>[30x]MSMYTTAQLLAANEQKFKFDPLFLRLFFRESYPFTTEKVYLSQIPGLVNMALY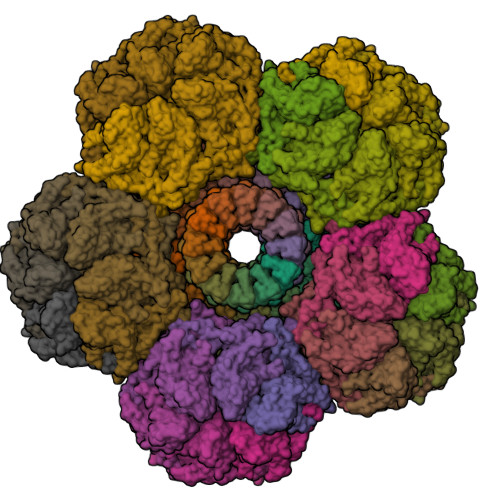VSPIVSGEVIRSRGGSTSEFTPGYVKPKHEVNPQMTLRRLPDEDPQNLADPAYRRRRIIMQNMRDEELAIAQVEEMQAVSAVLKGKYTMTGEAFDPVEVDMGRSEENNITQSGGTEWSKRDKSTYDPTDDIEAYALNASGVVNIIVFDPKGWALFRSFKAVKEKLDTRRGSNSELETAVKDLGKAVSYKGMYGDVAIVVYSGQYVENGVKKNFLPDNTMVLGNTQARGLRTYGCIQDADAQREGINASARYPKNWVTTGDPAREFTMIQSAPLMLLADPDEFVSVQLA;>[12x]MKTPTIPTLLGPDGMTSLREYAGYHGGGSGFGGQLRSWNPPSESVDAALLPNFTRGNARADDLVRNNGYAANAIQLHQDHIVGSFFRLSHRPSWRYLGIGEEEARAFSREVEAAWKEFAEDDCCCIDVERKRTFTMMIREGVAMHAFNGELFVQATWDTSSSRLFRTQFRMVSPKRISNPNNTGDSRNCRAGVQINDSGAALGYYVSEDGYPGWMPQKWTWIPRELPGGRASFIHVFEPVEDGQTRGANVFYSVMEQMKMLDTLQNTQLQSAIVKAMYAATIESELDTQSAMDFILGANSQEQRERLTGWIGEIAAYYAAAPVRLGGAKVPHLMPGDSLNLQTAQDTDNGYSVFEQSLLRYIAAGLGVSYEQLSRNYAQMSYSTARASANESWAYFMGRRKFVASRQASQMFLCWLEEAIVRRVVTLPSKARFSFQEARSAWGNCDWIGSGRMAIDGLKEVQEAVMLIEAGLSTYEKECAKRGDDYQEIFAQQVRETMERRAAGLKPPAWAAAAFESGLRQSTEEEKSDSRAA> MTTYLEFIQQNEERDGVRFSWNVWPSSRLEATRMVVPVAALFTPLKERPDLPPIQYEPVLCSRTTCRAVLNPLCQVDYRAKLWACNFCYQRNQFPPSYAGISELNQPAELLPQFSSIEYVVLRGPQMPLIFLYVVDTCMEDEDLQALKESMQMSLSLLPPTALVGLITFGRMVQVHELGCEGISKSYVFRGTKDLSAKQLQEMLGLSKVPLTQATRGPQVQQPPPSNRFLQPVQKIDMNLTDLLGELQRDPWPVPQGKRPLRSSGVALSIAVGLLECTFPNTGARIMMFIGGPATQGPGMVVGDELKTPIRSWHDIDKDNAKYVKKGTKHFEALANRAATTGHVIDIYACALDQTGLLEMKCCPNLTGGYMVMGDSFNTSLFKQTFQRVFTKDM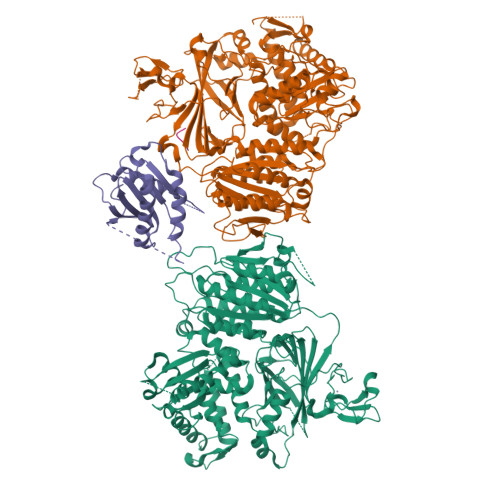HGQFKMGFGGTLEIKTSREIKISGAIGPCVSLNSKGPCVSENEIGTGGTCQWKICGLSPTTTLAIYFEVVNQHNAPIPQGGRGAIQFVTQYQHSSGQRRIRVTTIARNWADAQTQIQNIAASFDQEAAAILMARLAIYRAETEEGPDVLRWLDRQLIRLCQKFGEYHKDDPSSFRFSETFSLYPQFMFHLRRSSFLQVFNNSPDESSYYRHHFMRQDLTQSLIMIQPILYAYSFSGPPEPVLLDSSSILADRILLMDTFFQILIYHGETIAQWRKSGYQDMPEYENFRHLLQAPVDDAQEILHSRFPMPRYIDTEHGGSQARFLLSKVNPSQTHNNMYAWGQESGAPILTDDVSLQVFMDHLKKLAVSSA;> EGLRVVNLLQERNMLPSTPLKPPVPNLHEDIQKLNCNPELFRCTLTSIPQTQALLNKAKLPLGLLLHPFKDLVQLPVVTSSTIVRCRSCRTYINPFVSFLDQRRWKCNLCYRVNDVPEEFLYNPLTRVYGEPHRRPEVQNATIEFMAPSEYMLRPPQPPVYLFVFDVSHNAVETGYLNSVCQSLLDNLDLLPGNTRTKIGFITFDSTIHFYGLQESLSQPQMLIVSDIEDVFIPMPENLLVNLNESKELVQDLLKTLPQMFTKTLETQSALGPALQAAFKLMSPTGGRMSVFQTQLPTLGVGALKPREEPNHRSSAKDIHMTPSTDFYKKLALDCSGQQVAVDLFLLSGQYSDLASLGCISRYSAGSVYYYPSYHHQHNPVQVQKLQKELQRYLTRKIGFEAVMRIRCTKGLSIHTFHGNFFVRSTDLLSLPNVNPDAGYAVQMSVEESLTDTQLVSFQSALLYTSSKGERRIRVHTLCLPVVSTLNDVFLGADVQAISGLLANMAVDRSMTASLSDARDALVNAVIDSLSAYRSSVLSNQQPGLMVPFSLRLFPLFVLALLKQKSFQTGTNARLDERIFAMCQVKNQPLVYLMLTTHPSLYRVDNLSDEGALNISDRTIPQPPILQLSVEKLSRDGAFLMDAGSVLMLWVGKNCTQNFLSQVLGVQNYASIPQPMTDLPELDTPESARIIAFISWLREQRPFFPILYVIADESPMKANFLQNMIEDRTESALSYYEFLLHIQQQVNK;> MVLLTMIARVADGLPLAASMQEDEQSGRDLQQYQSQAKQLFRKLNEQSPTRCTLEAGAMTFHYIIEQGVCYLVLCEAAFPKKLAFAYLEDLHSEFDEQHGKKVPTVSRPYSFIEFDTFIQKTKKLYIDSRARRNLGSINTELQDVQRIMVANIEEVL;> EVTSII>[2x]AKVFQWFGSNESGAEFGSQNLPGVEGKDYIWPDPNTIDTLISKGMNIFRVPFMMERLVPNSMTGSPDPNYLADLI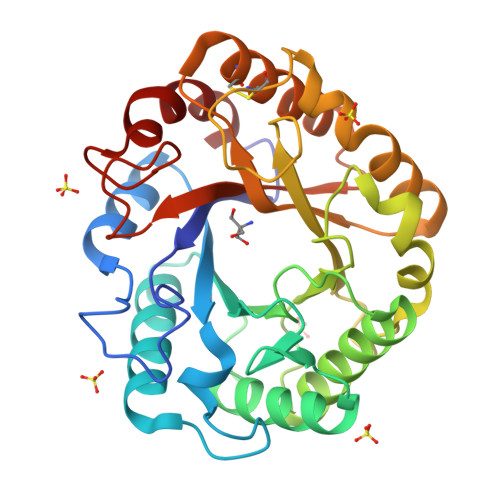ATVNAITQKGAYAVVDPHNYGRYYNSIISSPSDFQTFWKTVASQFASNPLVIFDTNNEYHDMDQTLVLNLNQAAIDGIRSAGATSQYIFVEGNSWTGAWTWTNVNDNMKSLTDPSDKIIYEMHQFLDSDGSGTSATCVSSTIGQERITSATQWLRANGKKGIIGEFAGGANDVCETAITGMLDYMAQNTDVWTGAIWWAAGPWWGDYIFSMEPDNGIAYQQILPILTPYL> ESSVNPVVLDFEDGT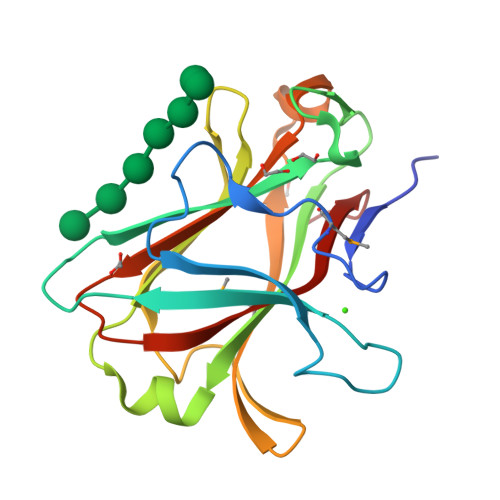VMSFGEAWGDSLKCIKKVSVSQDLQRPGNKYALRLDVEFNPNNGWDQGDLGTWIGGVVEGQFDFTGYKSVEFEMFIPYDEFSKSQGGFAYKVVINDGWKELGSEFNITANAGKKVKINGKDYTVIHKAFAIPEDFRTKKRAQLVFQFAGQNSNYKGPIYLDNVRIRPEDA>[4x]FNLDTEELTAFRVDSAGFGDSVVQYANSWVVVGAPQKITAANQTGGLYQCGYSTGACEPIGLQVPPEAVNMSLGLSLASTTSPSQLLACGPTVHHECGRNMYLTGLCFLLGPTQLTQRLPVSRQECPRQEQDIVFLIDGSGSISSRNFATMMNFVRAVISQFQRPSTQFSLMQFSNKFQTHFTFEEFRRSSNPLSLLASVHQLQGFTYTATAIQNVVHRLFHASYGARRDAAKILIVITDGKKEGDSLDYKDVIPMADAAGIIRYAIGVGLAFQNRNSWKELNDIASKPSQEHIFKVEDFDALKDIQNQLKEKIFAIEGTETTSSSSFELEMAQEGFSAVFTPDGPVLGAVGSFTWSGGAFLYPPNMSPTFINMSQENVDMRDSYLGYSTELALWKGVQSLVLGAPRYQHTGKAVIFTQVSRQWRMKAEVTGTQIGSYFGASLCSVDVDSDGSTDLVLIGAPHYYEQTRGGQVSVCPLPRGWRRWWCDAVLYGEQGHPWGRFGAALTVLGDVNGDKLTDVVIGAPGEEENRGAVYLFHGVLGPSISPSHSQRIAGSQLSSRLQYFGQALSGGQDLTQDGLVDLAVGARGQVLLLRTRPVLWVGVSMQFIPAEIPRSAFECREQVVSEQTLVQSNICLYIDKRSKNLLGSR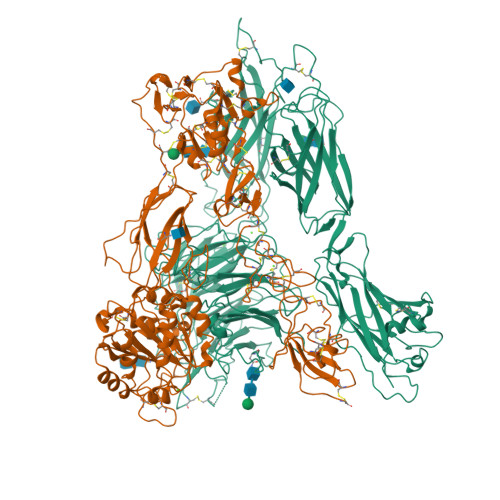DLQSSVTLDLALDPGRLSPRATFQETKNRSLSRVRVLGLKAHCENFNLLLPSCVEDSVTPITLRLNFTLVGKPLLAFRNLRPMLAADAQRYFTASLPFEKNCGADHICQDNLGISFSFPGLKSLLVGSNLELNAEVMVWNDGEDSYGTTITFSHPAGLSYRYVAEGQKQGQLRSLHLTCDSAPVGSQGTWSTSCRINHLIFRGGAQITFLATFDVSPKAVLGDRLLLTANVSSENNTPRTSKTTFQLELPVKYAVYTVVSSHEQFTKYLNFSESEEKESHVAMHRYQVNNLGQRDLPVSINFWVPVELNQEAVWMDVEVSHPQNPSLRCSSEKIAPPASDFLAHIQKNPVLDCSIAGCLRFRCDVPSFSVQEELDFTLKGNLSFGWVRQILQKKVSVVSVAEITFDTSVYSQLPGQEAFMRAQTTTVLEKYKVHGCGGLENLYFQ;>QECTKFKVSSCRECIESGPGCTWCQKLNFTGPGDPDSIRCDTRPQLLMRGCAADDIMDPTSLAETQEDHNGGQKQLSPQKVTLYLRPGQAAAFNVTFRRAKGYPIDLYYLMDLSYSMLDDLRNVKKLGGDLLRALNEITESGRIGFGSFVDKTVLPFVNTHPDKLRNPCPNKEKECQPPFAFRHVLKLTNNSNQFQTEVGKQLISGNLDAPEGGLDAMMQVAACPEEIGWRNVTRLLVFATDDGFHFAGDGKLGAILTPNDGRCHLEDNLYKRSNEFDYPSVGQLAHKLAENNIQPIFAVTSRMVKTYEKLTEIIPKSAVGELSEDSSNVVQLIKNAYNKLSSRVFLDHNALPDTLKVTYDSFCSNGVTHRNQPRGDCDGVQINVPITFQVKVTATECIQEQSFVIRALGFTDIVTVQVLPQCECRCRDQSRDRSLCHGKGFLECGICRCDTGYIGKNCECQTQGRSSQELEGSCRKDNNSIICSGLGDCVCGQCLCHTSDVPGKLIYGQYCECDTINCERYNGQVCGGPGRGLCFCGKCRCHPGFEGSACQCERTTEGCLNPRRVECSGRGRCRCNVCECHSGYQLPLCQECPGCPSPCGKYISCAECLKFEKGPFGKNCSAACPGLQLSNNPVKGRTCKERDSEGCWVAYTLEQQDGMDRYLIYVDESRECVAGPDGCGENLYFQ[4x]> MSEKKIIFVLIEHHGGKAHPVSWELIGKARDLASKLENSEVWGVLLGEGLESVAKEAIQ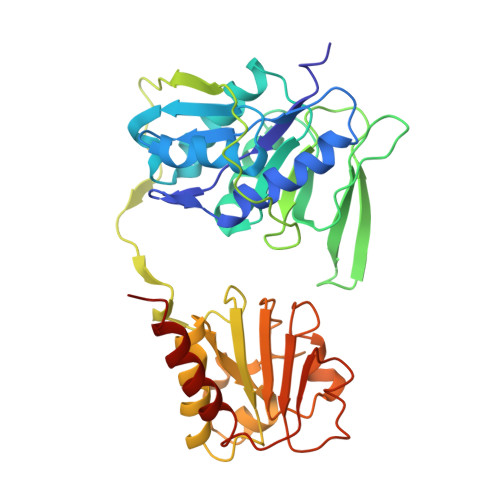RGADKVLYVKNREFNTYVNYLYKKALVDMVRKYRPEIFLIGATLEGRELAGMVATELETGLTADCTGLDIIPDKKLLAMTRPTFGGNLMATIMCPDHRPQMATVRPGVMKELPPDPERTGEIIEEEYDLGTFDKLIEILETIPLQTQVNLEYAPVVVAGGKGVGGPEGFKKLKELADLLGGEVGASRAAVKAGWISPEHQVGQTGKTVRPVLYFACGISGAIQHVVGIKESEIIVAINIDEKAPIFDIADIGIVGDLHKVVPALTAKLRELLNKSGVKK>MGSDKIHHHHHHMEVERLSLKEFCDMVAERKPTPGGGAVGSVVGAMACALAEMVANFTRKKKGYEDVEPEMERIVEAMEEARLKLFDLAKKDMEAFEKVMKAYKSSEGELQNALKEAASVPMDVIRVMKDLAHELEKLAEFGN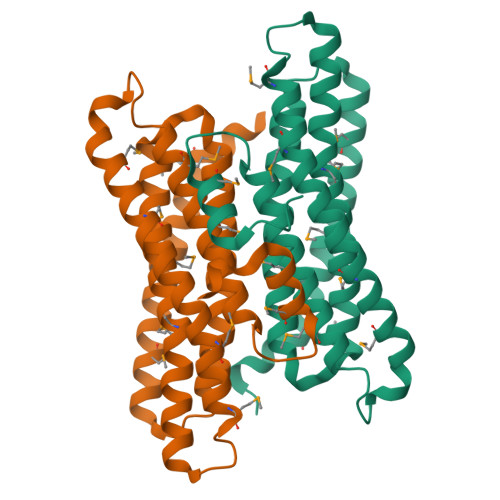KNLASDTLNAADLCHAVFQVEKVNVLINLKEISDETFRKNMLEELEEQEAQIEGCYQRVKKMLEGIVWSSK[2x]>[4x]TKPFTLPILTISELTNSRFPIPIEQLYTAPNENNVVQCQNGRCTLDGELQGTTQLLSSAVCSYRGRTVANSGDNWDQNLLQLTYPSGASYDPTDEVPAPLGTQDFSGILYGVLTQDNVSEGTGEAKNAKGVYISTTSGKFTPKIGSIGLH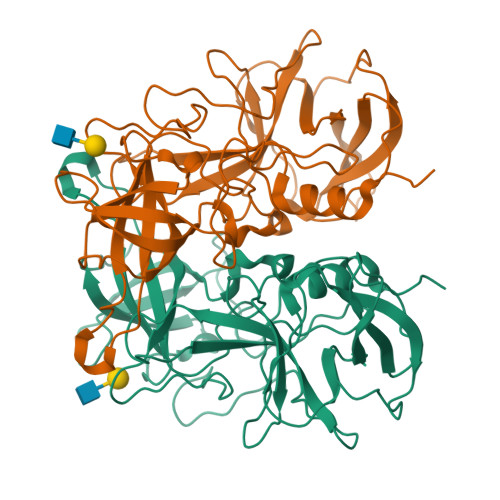SITENVHPNQQSRFTPVGVAQNENTPFQQWVLPHYAGALALNTNLAPAVAPTFPGEELLFFRSRVPCVQGLRGQDAFIDCLLPQEWVNHFYQEAAPSQADVALIRYVNPDTGRTLFEAKLHRSGFITVSHTGAYPLVVPPNGHFRFDSWVNQFYSLAPM>MNQSVSSLAEKDIQYQLHPYTNARLHQELGPLIIERGQGIYVYDDQGKGYIEAMAGLGSVALGFSNQRLIKAAEQQFNTLPFYHLFNHKSHRPSIELAEKLIEMAPVPMSKVFFTNSGSEANDTVVKFVWYLNNALGKPAKKKFISRVNGYHGVTVASASLTGLPGNQRGFDLPLPGFLHVGCPHHYRFALAGESEEHFADRLAVELEQKILAEGPETIAAFIGEPLMGAGGVIVPPRTYWEKIQKVCRKYDILVIADEVICGFGRTGQMFGSQTFGIQPDIMVLSKQLSSSYQPIAAILINAPVFEGIADQSQALGALGHGFTGSGHPVATAVALENLKIIEEESLVEHAAQMGQLL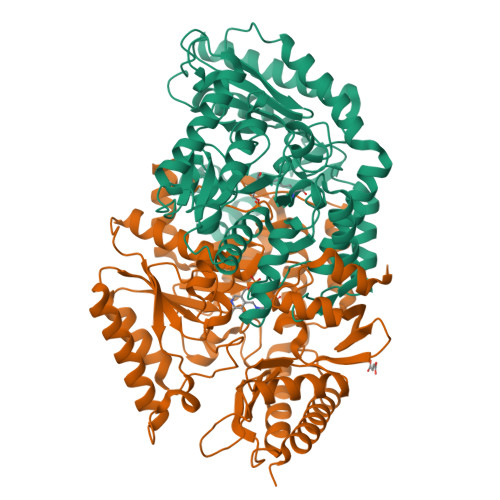RSGLQHFIDHPLVGEIRGCGLIAAVELVGDRVSKAPYQALGTLGRYMAGRAQEHGMITRAMGDAVAFCPPLIVNEQEVGMIVERFARALDDTTQWVGPGGHHHHHH[2x]>SADVAGAVIDGAGLGFDVLKTVLEALGNVKRKIAVGIDNESGRTWTAMNTYFRSGTSDIVLPHKVAHGKALLYNGQKNRGPVATGVVGVIAYSMSDGNTLAVLFSVPYDYNWYSNWWNVRVYKGQKRANQRMYEELYYHRSPFRGDNGWHSRSLG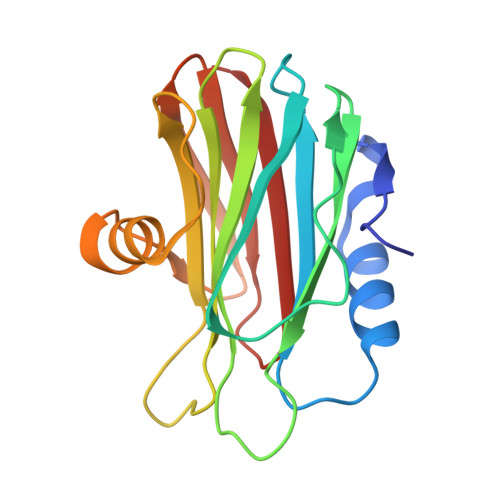YGLKSRGFMNSSGHAILEIHVTKA[2x]>[4x]MPDELKPHFANVQAHYDLSDDFFRLFLDPTQTYSCAYFERDDMTLQEAQIAKIDLALGKLGLQPGMTLLDVGCGWGATMMRAVEKYDVNVVGLTLSKNQANHVQQLVANSENLRSKRVLLAGWEQFDEPVDRIVSIGAFEHFGHERYDAFFSLAHRLLPADGVMLLHTITGLHPKEIHE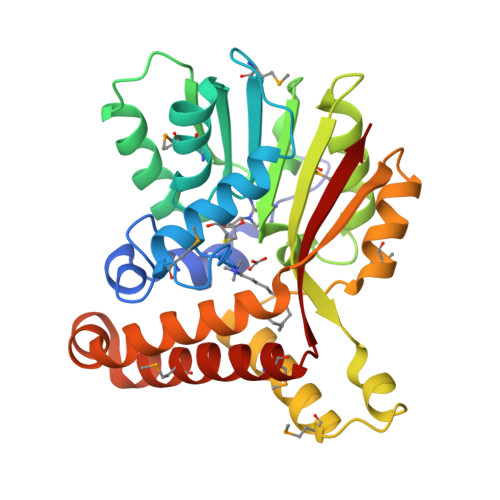RGLPMSFTFARFLKFIVTEIFPGGRLPSIPMVQECASANGFTVTRVQSLQPHYAKTLDLWSAALQANKGQAIALQSEEVYERYMKYLTGCAEMFRIGYIDVNQFTCQK>MEIGTVTSQEEKLAYEKSIEMAGNYANQFDAQMEANQAIARTLACTMAEYGSQDREEAMSIIKRILNENPQLIGVYLGYEPDAFDGRDKNYINAPGHDSTGRFVPYCNKINGPVIIEPLVHYDSSDYYQLPKTTGKDTLTEPYFYEGIFMVSYDSPIFKNGEFAGIAGVDVPLEYVDDVASSIRTFDTGYAFMVSNTGIFLSHPTQKNWIGEKSLSDFDVEEIKNAASDIREGIGGHVEIKDPITGKTVI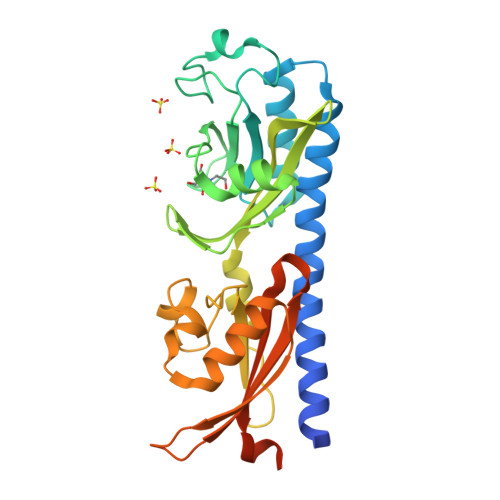MFYEPVKTGDFSFVLVVPKEEMLAGVKDLRDRLLEHHHHHH[2x]> MRENNTSFLVNVYDLKKFDTYAFNKVFIDDYKIFWINKGSAKLVDKNCLVSYTITASSVVLLKKNSIQRFSLMSLSDESISVCVLTIKNKFVNSLRHYLQGDLMIRNLYNEKKDLLLWNCELNDISVLGE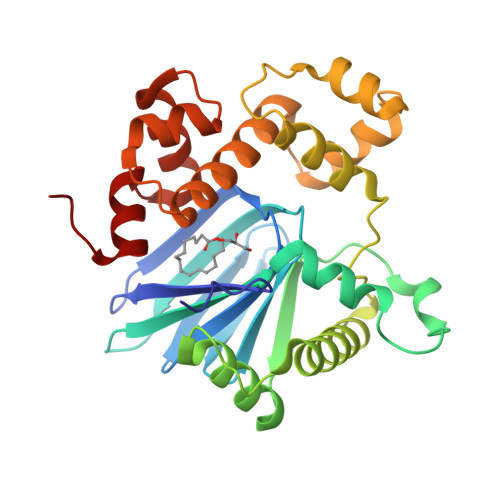IVSTYDQTQYSEDFLKIFFSGFFSKVEKKYNSIFITDDLDAMEKISCLVKSDITRNWRWADICGELRTNRMILKKELESRGVKFRELINSIRISYSISLMKTGEFKIKQIAYQSGFASVSYFSTVFKSTMNVAPSEYLFMLTGVAEE>MSKLTTGSFSIEDLESVQITINNIVGAAKEAAEKAEEELGPMGPTPFPTAATVRDWSFTLFDRYEPVYTPMCDQCCYCTFGPCNLEGNRRGACGLDMKGQAAREFFLRCITGCACHSAHGRHLLDHIISIFGEDMPINMGASNVIAPNIQLITGRQPKTLGDLKPIMEYVEEELGQLLATVHAGQEGAAIDYDNKAMLAGILDHVGMEVSDIAQVTALGFPKSDPEAPLVEVGMGTLDASKPVIIAIGHNVAGVTYIMDYMEDNNLTDKMEIGGLCCTAFDMTRYKREDRKPPYAKIVGTISKELKVVRSGIPDVIVIDEQCVRADLVEEGKKLKIPVIASNEKVMYGLPDRTNDDVDAIIEDIKTGKIPGCVMLDYEKLGELVPRLAMEMAPLREGISAIPSDEEMASLVAKCVACGECALACPEELDIPDAIQAAKEGDFTALDFLHDLCVGCRRCEQVCNKEIPILSVIDKAAQKAIAEEKGLVRAGRGQVSDAEIRAEGLNLVMGTTPGVIAIIGCANYPAGSKDVYRIAEEFLNRNYIVAVSGCSAMDIGMYKDADGKTLYERFPGRFERGNILNTGSCVSNSHISGTCHKVAAIFAGRNLSGNLAEIADYTLNRVGAVGLAWGAYSQKAAAIGTGCNMYGIPAVLGPHSGKYRRALIAKTYDENKWKVYDSRNGSELDIPPSPEFLITTAETWQEACVLLAKNCIRPSDNNMGRSIKLTHWIELSEKYLGVLPEDWWKFVRHEADLPLSRREELLKKLETEHGWEIDWKKKKIISGPKIKFDVSSQPTNLKRLCKEA[2x];>[2x]MVDTTKNTKLFTSYGVKTSKAITTEVAAKLISKAKRPLFVVGTGVLDPELLDRAVKIAKAKNIPIAATGSSMPGFVDKDVNAKYINLHQLGFYLTDPDWPGLDGNGNYDTIILLGHKKYYINQVLSAVKNFSDVKSISIDRNYIQNATMSFGNLSKADHIAALDEVIDLL

Carbon monoxide dehydrogenase (CODH) and acetyl-CoA synthase (ACS) play major roles in the global carbon cycle through the consumption of CO and CO2 gases, production of acetate, and breakdown of acetate for methane generation. By contrast, methanogenic archaea employ four copies of CODH (α2ε2 heterotetramers) and eight copies of ACS (β monomers) that interact stably with eight copies of CFeSP (γδ heterodimers) to form a massive 2.2 MDa complex called the acetyl-CoA decarbonylase/synthase (ACDS) complex. ACDS plays a central role in that process, wherein the A-cluster of ACS cleaves acetyl-CoA into CO and a methyl moiety, the C-cluster of CODH oxidizes CO to CO2, and the corrinoid of CFeSP receives the methyl moiety, which is reduced to methane in downstream methanogenic metabolism. Through plunge freezing of the ACDS complex, we captured multiple subcomplexes including a CODH tetramer, a CODH/ACS pentamer, and a CODH/ACS hexamer and characterized these subcomplexes via cryogenic electron microscopy (cryo-EM).

With the next-generation chameleon instrument, different dissociation behavior led to formation of (α2ε2)β and (α2ε2)β2 CODH/ACS subcomplexes in addition to the α2ε2 CODH subcomplexes, allowing us to capture methanogenic CODH/ACS subcomplexes. The use of two plunging methods allowed us to capture two snapshots of MetCODH, with global resolutions of 2.8 and 3.3 Å for the maps from chameleon and Cp3-plunged samples, respectively. The MetCODH α2ε2 heterotetramer shares the same topology as MebCODH and harbors the same set of metallocofactors, including E- and F-clusters, which are not present in monofunctional and acetogenic CODHs. Even in our chameleon-plunged specimen, most of the observed CODH particles did not have ACS bound. In the structures of MetCODH without ACS bound, this CO channel is closed. The structural basis for channel closing appears similar to that previously observed for MoorCODH/ACS. In both cases, helix αA shifts toward helix αB to close the gas channel and block CO release. Instead of Val507(Met)/Val149(Moor), Leu504(Met)/Ile146(Moor), and Phe601(Met)/Phe229(Moor) creating an alcove for bound-CO, these residues now create a choke point in the CO channel. Additionally, helix αA residue Arg500(Met)/Arg142(Moor) has repositioned so that it no longer hydrogen bonds to the A-cluster coordinating Gly279(Met)/Gly596(Moor).>GPSSPSLLRAIPGIAWIALLLLVIFYVFAVMGTKLFAQSFPEWFGTLGASMYTL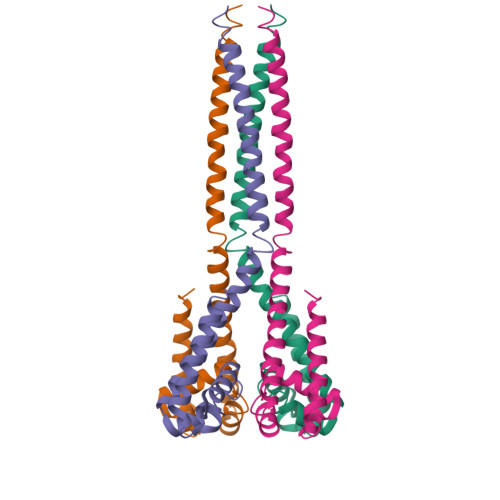FQVMTLESWSMGIARPVIEAYPWAWIYFVSFILVSSFTVLNLFIGIIIESMQSAHWEAEDAKRIEQEQRAHDERLEMLQLIRDLSSKVDRLERRSGKR[8x]> MQFFKTLAALVSCISFVLAYVAQDVHVSFPSTAGKSRVMIGKVEPRIGIDETVPTTITVEDPNEVIQVNFAIESTNKPFQNTLLIGLPNKNLEMAFEPEIKDNGKLSMYKYRIDLAKLDAALLQEASRSPEPIKATLILASSTAKPKENLFREILQLNLNFDVDHSDSSLVDKFGIKPEIHHIFHAEPKRVAKPIAVIFVLII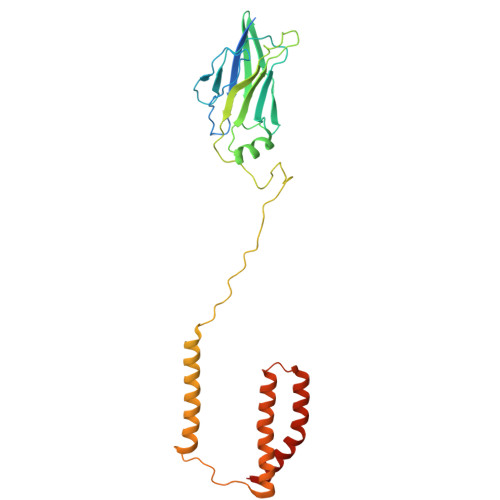FITILSLIVTWLNSCAAAFNNIPTGVTAVYFLGFIATIVGFEVIFARYYLGTSIFETLFSSLYLGAPGLLTSTKFLRSFGQTI> SKETKPLPDYVAWKDADALIVHSDKTLETKRSEFGTSIITPEEKLYIRNNVNTPPESILADRDGWKVEISGVKEPRTLTVAELKTLGLVTAATVLQCSGNGRKYFKDQLTGDQKMSGTPWTVGAAGCVIWSGVPLKAVVDALGGPAEGARFITGTGGEELPAGLDPKLLVVERSVPISNLDNVILAWEMNGRPLSLAHGGPLRMVVPGYSGVNNIKYVKAVAM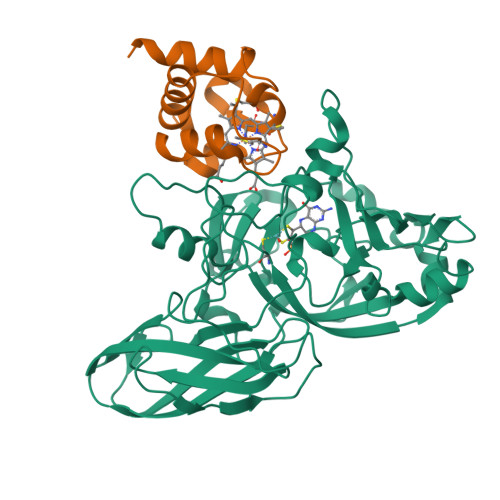TEVETDAKIQKTSYRVHALGEKGSPDQPSVWEQPVKSWITTPHEAAKAGQVQIAGVAFGGMNACKSVEVSVDGGQTWQEAEFIGPDLGRFAWRVFALSADLARGTYTLVSRATDTEGNVQPEETEMNGAGYGHNGWRAPAVKLTVA;> MEEDKLALGREIFLERSEPQCALCHTLADAEAVGEVGPNLDELKPDAERVNTAVTNGIGPMPANEILTDEEIEAVALYVSTVAGKAKNSSSVDKLAAALEHHHHHH> MNQKAVILDEQAIRRALTRIAHEMIERNKGMNNCILVGIKTRGIYLAKRLAERIEQIEGNPVTVGEIDIT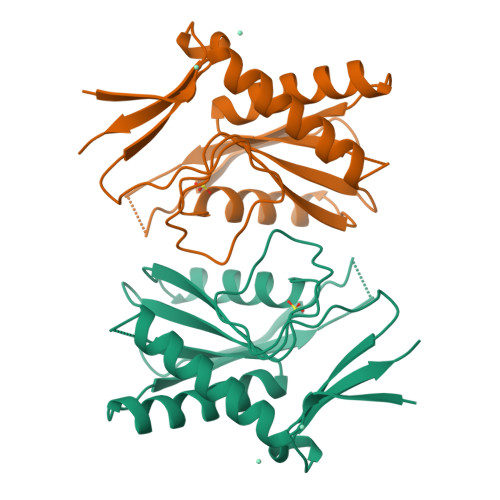LYRDDLSKKTSNDEPLVKGADIPVDITDQKVILVDDVLYTGRTVRAGMDALVDVGRPSSIQLAVLVDRGHRELPIRADYIGKNIPTSKSEKVMVQLDEVDQNDLVAIYENE> MFEVKMGSKMCMNASCGTTSTVEWKKGWPLRSGLLADLCYRCGSAYESSLFCEQFHKDQSGWRECYLCSKRLH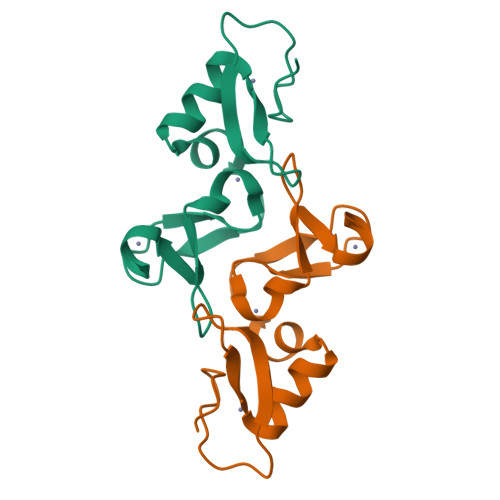CGCIASKVTIELMDYGGVGCSTCACCHQLNLNTRGEN>[8x]MCDIGLIGLAVMGQNLSLNISSKGFKIGVYNRTYERTEETMKRAKEENLVVYGYKTVEELINNLKKPRKVILLIKAGPAVDENISNILKHFEKG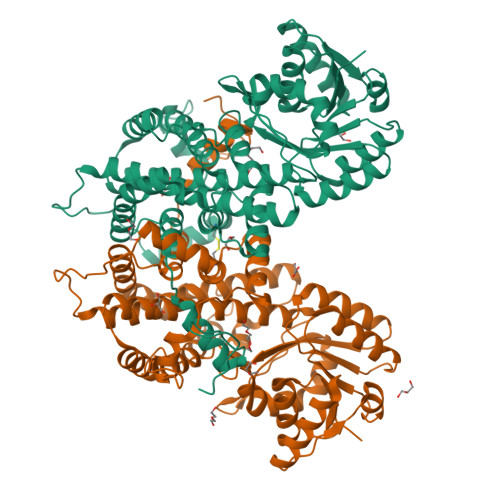DIIIDGGNEWYINSERRIKLCKEKDVEYLAMGVSGGEAGARYGCSFMPGGSKYAYDCVKEILEKCSAQVGNSPCVTYIGPGSSGNYVKMVHNGIEYGDMQLISESYVIMKHILKYDNQKLSEVFNKWNEGILNSYLIEITANILAKKDDLTNNYLVDMILDIAGAKGTGKWTMLEATERGIPCPTMCAALDARNISVFKELRTKAESNFNKDNILIDPNEDLNDFENDLLNALYCCKIISYTQGLFLLKQVSEEMNWKLNLGEIARIWRGGCIIRAVFLDRIANAYKNNEKLELLFLDNEFSDDIKNKLPSLRKIVLMATKYSIPIPAFSASLAYFQMVTSQNLPLNLVQAQRDYFGSHTYRRTDREGNYHTLW>SNAFAEDNSAALDTLVQTEARKVMQENNITGLSIAITRHGKQQFYNYGVASKATGQPVSSDTLFELGSISKTFTATLATWAQANGRLSLTQSIDTYMPPLRDTRLGKIPVFHLGTHTAGGFPIQVPEKVQNTRQLMDYFKAWQPEYLPGTHRTYANPSIGLLGVIAARSMNMPFQEAMQQRLFPALGLNSTYVNVPDDKQTLYAQGYNTLDEPVRVNPGILAAEAYGVKSSSRDLIRFVEANIGLGQYDAPLQRALSDTRIGYFKVGGMTQDLAWEQYPTPIHLDVLL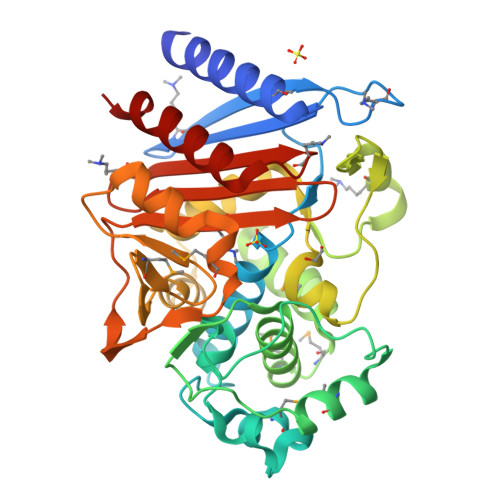AGNASAMLNTQKADAIEPPLAAQPTAWVNKTGSTNGFGGYVAFIAQKQLGIVILANKNYPNEERVKLAYRILQHAEPL[4x]1-benzyl-3-tert-butyl-1H-pyrazole-5-carboxylic acid | C15 H18 N2 O2 | 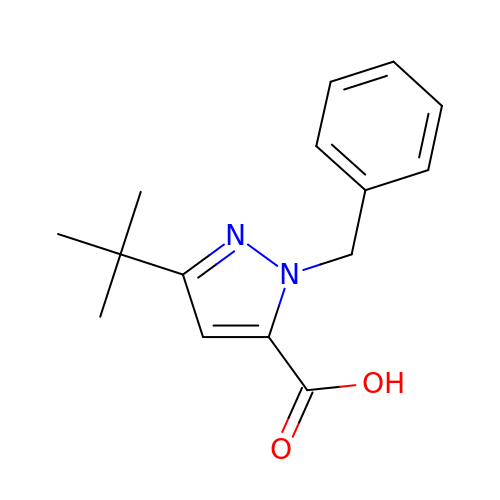IJXYLILRNVOJNF-UHFFFAOYSA-N> MAKRKAEDTQSDKMATAEKVAQNDYTIGLVDPVKDY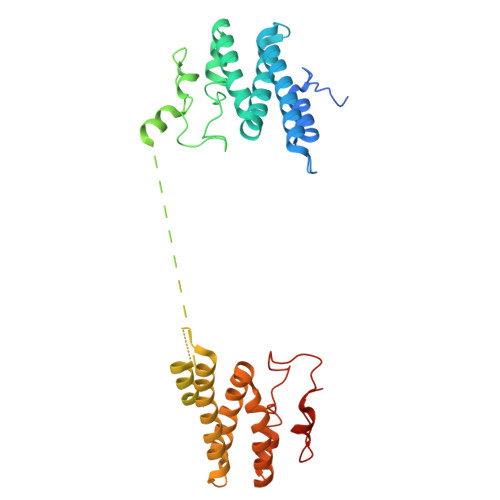QKLIETRVQVDEIVDDDVTKENFDRTAAAARDVIWRLLFDEAGTSQSNTEKASQLLEEYRGDACFYDPTPYNEWIVKLRDEVLKKELLDFWRDVLVKKQLGPCWSRDSDLFDSDDTPPLEFYAHAGCTAPFAASLKVRAALEEQASLDQDGPATPTTPGELSADDAAALSGEFEATLTKENPLEEYRTLMKRFVLTKIIVPDSVHQASVKKIAAAAREIIWKLLFDGTPSAEDQNKAAELLQEYKGDAGFYGPDDYNSWIFNLRDEVLTKELLDFWRDKMVKMELGPSCARDSDYYDNEDPLPFEFYEKAGCKAPFEGPVNDD> APAILLVDDEPHSLAAMKLALEDDFDVLTAQGAEAAIAILEEEWVQVIICDQRMP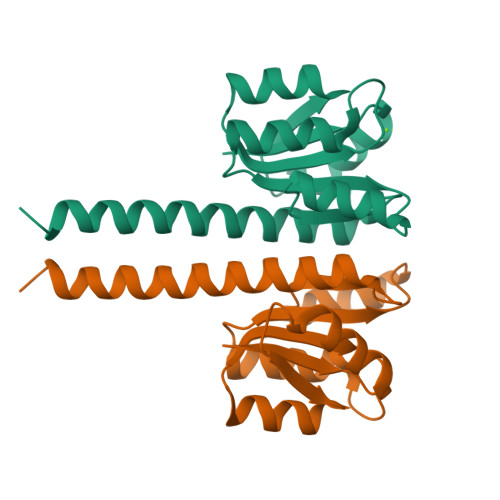GRTGVDFLTEVRERWPETVRIIITGYTDSASMMAAINDAGIHQFLTKPWHPEQLLSSARNAARMFTLARENERLSLEMRLLERP>SGLVPRGSHMQKDFWLSEIGDKNISLGYYDDNVAIVLTNKTDKILRVYSYEDGKIRKDFEQKEIITGLMGDKKIEGDLKTPVGFYELGRKFNPGDPYYGPFAFATTYPNLLDKVQGKTGGGIWIHGYPLDGSRLDEFKTRGCIALFNNNLEKFAQVVQDKKVFVMTEEKEKIRAKKDQIASLLADLFTWKLAWTNSDTNTYLSFYDEQEFKRFDKMKFEQFASMKKSIFSRKEDKKIKFSDINISPYPNLENETMYRISFYEDYYTKNYQFRGDAILYVKIDSKGKMKILAEQ[2x]

The helical morphology of Campylobacter jejuni, a bacterium involved in host gut colonization and pathogenesis in humans, is determined by the structure of the peptidoglycan (PG) layer. Pgp2 is an LD-carboxypeptidase that cleaves D-Ala from both monomeric and cross-linked tetrapeptides. The structure of Pgp2 contains an N-terminal helix (residues Q43-I51), the catalytic LD-CPase domain (residues V65-K201), and the C-terminal NTF2 domain (residues K208-Q325), each connected to the next domain by a single loop. In summary, we show that helical shape in C. jejuni depends on both the LD-CPase and NTF2 domains of Pgp2.

The K307A variant (Pgp2K307A), a conserved residue within the pocket of the NTF2 domain, was also weakly associated, supporting a role for this binding pocket for appreciable PG interaction. To investigate if the loss of PG binding by the Pgp2K307A was due to conformational change, the crystal structure of this variant was solved at 1.85 Å resolution. The Pgp2K307A crystal structure contains two Pgp2K307A molecules in one asymmetric unit that superimposed with an RMSD of 0.7 Å over 281 Cα atoms. The fold of the Pgp2K307A is similar to that of wild-type Pgp2 (RMSD of 1.5 Å over 277 aligned Cα atoms). The largest deviation is located at residues 296–306 of strands β9–β10, which form a protruding lower lip of the NTF2 domain binding pocket. We conclude that β9–β10 is conformationally flexible and may allow variation in ligand specificity. In addition, we used two Pgp2 crystal structures (WT and Pgp2K307A) as initial docking conformers. The catalytic triad mutants (C174S, H157A) and three mutants within the NTF2 pocket (Y233A, K257A, and K307A) resulted in bacteria with cell curvature distributions that were similar to the Δpgp2 strain. Lower levels of products were observed in the NTF2 domain mutant strains (K257A, K307A, and E324Q) relative to the strain expressing wild-type Pgp2. Pgp2 but not the K307A mutant was pulled down by C. jejuni Δpgp2 PG sacculi, supporting a role for the pocket in PG binding.> REARGATEEPSPPSRALYFSGRGEQLRLRADLELPRDAFTLQVWLRAEGGQRSPAVITGLYDKCSYISRDRGWVVGIHTISDQDNKDPRYFFSLKTDRARQVTTINAHRSYLPGQWVYLAATYDGQFMKLYVNGAQVATSGEQVGGIFSPLTQKCKVLMLGGSALNHNYRGYIEHFSLWKVARTQREILSDMETHGAHTALPQLLLQENWDNVKHAWSPMKDGSSPKVEFSNAHGFLLDTSLEPPLCGQTLCDNTEVIASYNQLSSFRQPKVVRYRVVNLYEDDHKNPTVTREQVDFQHHQLAEAFKQYNISWELDVLEVSNSSLRRRLILANCDISKIGDENCDPECNHTLTGHDGGDCRHLRHPAFVKKQHNGVCDMDCNYERFNFDGGECCDPEITNVTQTCFDPDSPHRAYLDVNELKNILKLDGSTHLNIFFAKSSEEELAGVATWPWDKEALMHLGGIVLNPSFYGMPGHTHTMIHEIGHSLGLYHVFRGISEIQSCSDPCMETEPSFETGDLCNDTNPAPKHKSCGDPGPGNDTCGFHSFFNTPYNNFMSYADDDCTDSFTPNQVARMHCYLDLVYQGWQPSRKPAPVALAPQVLGHTTDSVTLEWFPPIDGHFFERELGSACHLCLEGRILVQYASNASSPMPCSPSGHWSPREAEGHPDVEQPCKSSVRTWSPNSAVNPHTVPPACPEPQGCYLELEFLYPLVPESLTIWVTFVSTDWDSSGAVNDIKLLAVSGKNISLGPQNVFCDVPLTIRLWDVGEEVYGIQIYTLDEHLEIDAAMLTSTADTPLCLQCKPLKYKVVRDPPLQMDVASILHLNRKFVDMDLNLGSVYQYWVITISGTEESEPSPAVTYIHGSGYCGDGIIQKDQGEQCDDMNKINGDGCSLFCRQEVSFNCIDEPSRCYF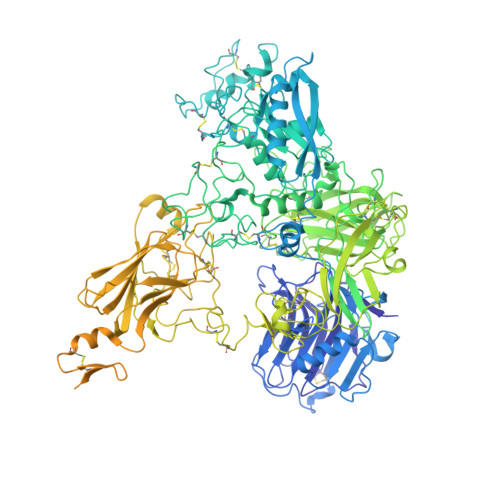HDGDGVCEEFEQKTSIKDCGVYTPQGFLDQWASNASVSHQDQQCPGWVIIGQPAASQVCRTKVIDLSEGISQHAWYPCTISYPYSQLAQTTFWLRAYFSQPMVAAAVIVHLVTDGTYYGDQKQETISVQLLDTKDQSHDLGLHVLSCRNNPLIIPVVHDLSQPFYHSQAVRVSFSSPLVAISGVALRSFDNFDPVTLSSCQRGETYSPAEQSCVHFACEKTDCPELAVENASLNCSSSDRYHGAQCTVSCRTGYVLQIRRDDELIKSQTGPSVTVTCTEGKWNKQVACEPVDCSIPDHHQVYAASFSCPEGTTFGSQCSFQCRHPAQLKGNNSLLTCMEDGLWSFPEALCELMCLAPPPVPNADLQTARCRENKHKVGSFCKYKCKPGYHVPGSSRKSKKRAFKTQCTQDGSWQEGACVPVTCDPPPPKFHGLYQCTNGFQFNSECRIKCEDSDASQGLGSNVIHCRKDGTWNGSFHVCQEMQGQCSVPNELNSNLKLQCPDGYAIGSECATSCLDHNSESIILPMNVTVRDIPHWLNPTRVERVVCTAGLKWYPHPALIHCVKGCEPFMGDNYCDAINNRAFCNYDGGDCCTSTVKTKKVTPFPMSCDLQGDCACRDPQAQEHSRKDLRGYSHG>GSHMLSTGDNLE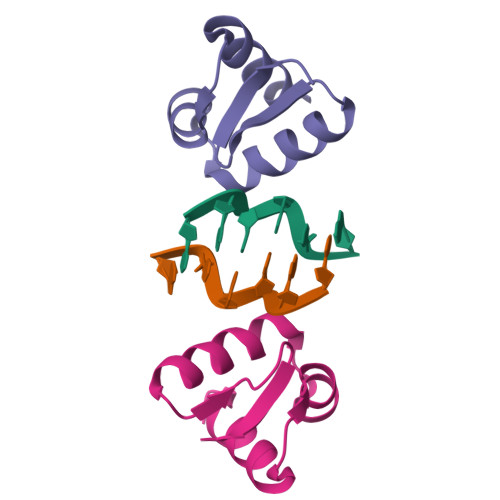QKILQVLSDDGGPVAIFQLVKKCQVPKKTLNQVLYRLKKEDRVSSPSPKYWSIGG[2x]>MRDLDREETYLVDRTGLALELRDLVGTGPVPGEAYPGPHAALGYGEGQFAALLSGLPDWGEEGTLFLLEGGYDLGEAAGMALLAETGRARVVRVGFRPGVEVHIPPSPLAPYRYLRFLLLATGREEVLRSVDEALLEERRRLGPEVPVEENPAKFLAYTLLERLPLFYSPLFRPLEGAVQTLFARVAKSLSLTPPPSALEFFLVGLEARHEQGDPLAAVLLGPGEEAALAKEILESRVDALAEVPATGANRLAQVMALWYRMAWTAYYLALLYGVDPGD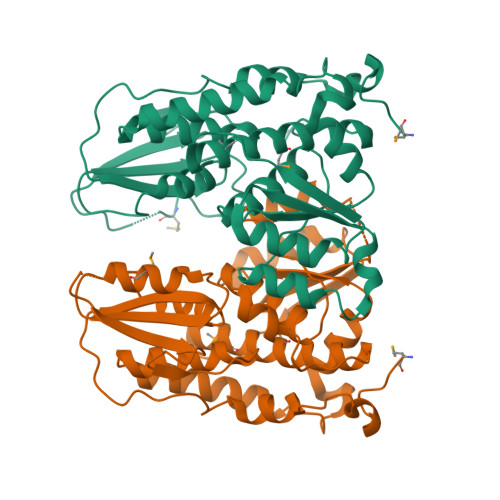HGLLERLREVT[2x]> MESGIDLQGQFISALQSLGLSHDLAKLLWLPLPMLMMLIVATVGVLVAVWLERKISAAVQQRIGPEYIGPLGILAPLADGLKLIFKEDVLPANSDRWLFTLGPAVVVIPVFLSYIIVPFGQNLLISNLAMGVFLWIALSSIAPIGLLMAGYASNNKYSLLGGLRAAAQSISYEIPLALAVLAVAMMSNGLGTVEIVEQQSQYGILSWNVWRQPIGFLVFWIAALAECERLPFDLPEAEEELVAGYQTEYAGMKFALFYLGAYVNLVLSALLVSVLYFGGWSFPIPLETIANLLGVSETNPFLQIAFAVLGITMTLIKAYFFVFLAILLRWTVPRVRIDQLLDLGWKFLLPVGLVNLLLTAGLKLAFPVAFGG;> MDLVTLAGQLNAGTILPETILIVTLLVVLLADLIQGRQADRWTPYFAIVGLGGAIATMIPLWTQPATISFFGSFISDHLSLFFRGLIALSALGTILMSIRYVEQTGSSLGEFMTILLTATVGGMFIAGAQELVFIFVALETLSIASYLLTGYTKRDSRSNEAALKYLLIGAASSAIFLYGSSLLYGLSGGHTQLPAIAQALSSESLGLVVALVFVIAGISFKISAVPFHQWTPDVYEGAPTPVVAFLSVGSKAAGFALAIRFLTLAFPSVTDQWQLIFTVLAILSMILGNVVALAQTSMKRMLAYSSIGQAGFVMIGFVVGTEAGYASMLFYLLVYLFMNLGAFTCVILFSLRTGTDQISEYAGLYQKDPLLTLGLSLCLLSLGGIPPLAGFFGKIYLFWAGWQAGAYGLVLLGLLTSVISIYYYIRVVKMMVVKEPQEMSEAVRNYPEVSWSSFGLRPLQVGLVMTVIATSLAGILANPLFNLVNTAVWDVPQLANQPTVMEVAYQALSPAGKS;> MVAIPRLRDTATVFVLSGYEYFLGFLIICSLVPVLALAASALLRPKSGRMIRLTTYESGMEPIGGAWIQFNVRYYMFALVFVIFDVETVFLYPWAVAFHQLGLLAFIEALIFIAILVVALVYAWRKRALEWS;> MSTFPWLTTIILFPIVAALAIPFIPDPTGKGRPIRWYALAVGLIDFALIVYAFTNFYDLNTPGMQLWESYDWIPEIGLRWSVGADGLSMPLILLTGFITTLAILAAWPVTLKPRLFYFLMLAMYGGQIAVFAVQDMLVFFLAWELELIPVYLLLAIWGGHKRQYAATKFILYTAGSSLFILVAGLAMAFYGDTVSFDMQTLAAKDYALGFQLLVYAGFLVAYGVKLPIVPLHTWLPDAHGEATAPVHMLLAGILLKMGGYALIRMNVDMLPAAHAKFAPVLVILGVVNIIYAALTSYAQRNLKRKIAYSSISHIGFVLIGIASFTNLGMSGAVLQMVSHGLIGASLFFLVGATYDRTHTLILEEMGGVGQKMKKIFAMFTACSLASLALPGMSGFVAELMVFIGFATSDAYSLPFRVIVVFLAAVGVILTPIYLLSMLREIFYGPENKELVEHEALVDAEPREVFIIACLLVPIIGIGLYPKLLTQIYDATTGQVIARAREVLPTLAQQTEQPLGILPMVAPQLKANAQ;> MQLTYVLILAALLFCIGIYGLVTSRNAVRVLMSIELLLNAVNLNLIGFANYLDGQQIKGQVFAVFVITVAAAEAAVGLAIILAIYRNRDTVDMEKFNLLKW;> MEPLYQYAWLIPVLPLLGALIVGFGLIAFSETTSKLRRPSAIFIMALMAIAMGHSLTLFWSQVQGHLPYTQMIEWAAAGNLHIAMGYVIDPLAALMLVIVTTVAFLVMLYSDGYMAHDPGYVRFFAYLSLFGSSMLGLVVSPNLVQVYIFWELVGMCSYLLIGFWYDRKSAAEAAQKAFVTNRVGDFGLLLGMVGLFWATGTFDFAGMGDRLTELVNTGLLSPSLAAILAILVFLGPVAKSAQFPLHVWLPDAMEGPTPISALIHAATMVAAGVFLIARMFPVFEQLPQVMTTIAWTGAFTAFMGATIAITQNDIKKSLAYSTISQLGYMVMGMGVGAYSAGLFHLMTHAYFKAMLFLGSGSVIHSMEGVVGHNPDLAQDMRYMGGLRKYMPITGATFLVGCLAISGVPPFAGFWSKDEILGAVFHANPAMWLLTWLTAGLTAFYMFRMYFMTFEGKFRNVPPERQEHHDHHSHHAAVPHESPWTMTLPLVVLAIPSTLIGFVGTPFNNLFEVFIHAPGEEKVAEHAVDLTEFLILGGSSVGIGLMGITVAYLMYLKGTPSPQAIAKAIQPLYQFSLHKWYFDELYEAVFIKGCRRLARQVLEVDYNVVDGVVNLTGFVTMVTGEGLKYLQNGRAQFYALIVLLAVLGFVIFSVQT;> MDLATLTQTITFFALAAAVIIAALGVVLLDNVVYSAFLLGGVFLSIAGLYILMNADFVSAAQILIYVGAVNVLILFAIMLVNKRETYTPVPGRWLRQGGAAVVSLGVFALLTKMILQTPWQLSSVPPTPDSITTIGQHFFSDFLLPFELASVLLLMALIGAVVLARRELVLEPEPILGEEVVPPLELPERPREPVALSEK;> MPKIETRTEPMVINMGPHHPSMHGVLRLMVTLDGEDVIDCEPVIGYLHRGMEKIAENRTNIMFIPYVSRWDYAAGMFNEAVTVNAPEKLAGIPVPKRASYIRVIMLELNRIANHLLWLGPFLADVGAQTPFFYIFREREYIYDLFEAATGMRFINNNYFRIGGVAADLTYGWVTKCRDFCDYFLPKVDEYERLITNNPIFVRRLQGVGKISREEAINWGLSGPMLRASGVKWDLRKVDHYECYDDFDWDVPVATEGDCLARYIVRIQEMRESVKIIRQALDGLPGGPYENLEAKRMLEGAKSEWNGFDYQYIGKKLSPTFKIPKGEHYVRVESGKGELGIYLIGDDNVFPWRWKIRPPDFNNLQVLPQLLKGMKVADIVAILGSIDVIMGSVDR;> MKFLNQITNYAKEAVQSAKYIGQGLSVTFDHMRRRPITVQYPYEKLIPSERFRGRIHFEFDKCIACEVCVRVCPINLPVVDWVFNKELKKKELKHYSIDFGVCIFCANCVEYCPTNCLSVTEEYELATYDRHELNYDSVAMGRIPYKVTQDPMVTPIREFAYLPAGVMSGHDLPAGAQRAGERPEAIANTAKSSEN;> MSDTPEAPIVEAGPVGRLLQSQNLSVESLGRDASGVEMIKVDRDRLLAVCQTLYADGFNYLRCQAAYDSGPGQDLVSTYHLIKLSDNADRPPEVRIKVFVPRDDPRVPSVYWIWKTADWQERESYDMFGIVYEGHPNLKRILMPEDWVGWPLRKDYITPDFYELQEAY;> MTNTTSPAILNPIARPEVPQELAENIILTSLNDVYDWARLSSLWPLMYGTACCFIEFAAMIGSRFDFDRFGLVPRNSPRQADLIITSGTITMKMAPALVRLYEQMPSPKYVIAMGACTITGGMFSSDSYSAVRGVDKLIPVDVYLPGCPPRPEAIMDAIVKLRKKIANEHINERGNLAQTHRLFTAKHKMKPVPPILTGQYLNAPSRQAPPPALAAAMGIAVPALGEAVSETTSVAE;> MAVSTELLVLGVYGALAGLYLLVVPAIVYAYLNARWYVASSFERAFMYFLVTFFFPGLLLLAPFINFRPQPRSLNS;> MLLKSTTRHVHIYAGHVVDGEVHPDTETLTLNVDPDNELEWNEAALAKVEAKFRELVANAAGEDLTEYNLRRIGSDLEHFIRSLLMQGEIGYNLNSRVRNYSLGIPRVNHS;> MGLLAGYQFVKDLESAGALALFVPPEGGFEGRYQRRLRSKGYTTLPMSAPGLGDLAAYLTQEHGIRPAHTGKEDIRVYFQPPLVTYHLENLPPNAKGLVLWLIDGKRLSKQEFAYLAQLTQTLPKFKVVVEVGGDRVVRWEPLADWVAAA;> MAIKKGDLVKVVAEKLANSLEALASDHRYPPYLFEGRGEVVDIRGDYAQIKFPVPTPTVWLRLDQLEVAQ;> MDAVISVKPILLAMTPVFILLCLFFGTRNGFYDTDQYHGNGSAH;> MATDFNRGIMKFDGADSPAMIAISAVLILGFIAALIWWALHTAYA;> MIRPIADTYPLLPLSKAQMGQRQEIINSHKRLWDKTMATDLIMTILPGMTVKVTNPNDTYYQFQGIVQRITDGKVAVLFEGGNWDKLVTFQASELEPVVVTPKEKAKAKK

In both cyanobacteria and plants, a type-I NAD(P)H dehydrogenase-like (NDH-1) complex is crucial for CEF and respiration. The NDH-1 complexes belong to the NAD(P)H:Quinone oxidoreductase family that includes the complex I (NADH dehydrogenase) of the respiratory chain in bacteria and mitochondria. The electron delivered from Fd is eventually transferred to PQ which is bound within the NDH complex. To further advance our understanding of NDH functionality, we solved two single particle cryo-electron microscopy (cryo-EM) structures of NDH-1L from T. elongatus BP-1.

We first solved the structure of NDH-1L complex purified from T. elongatus BP-1 at an overall resolution of 3 Å. Interestingly, we found that the NDH-1L complex binds a PQ molecule at a pocket above the membrane plane. We assume that this is an endogenous PQ molecule, which was trapped in the cyanobacterial NDH-1L complex during purification, as was earlier reported for Escherichia coli complex I40. Thus, we named this structure as NDH-PQ. Similar to the two previously reported cyanobacterial NDH-1L structures, our NDH-PQ structure also contains 18 subunits, without any signs of association with NdhV. In addition, we found that the NdhS subunit in the NDH-PQ structure exhibits weak cryo-EM density, suggesting that NdhS is also loosely associated. In the NDH-PQ structure, we modeled a PQ molecule in a pocket (PQ chamber) at the interface of the membrane and hydrophilic arms. The smaller PQ chamber is caused by the different conformation adopted by the β1-2 loop of NdhH, which intrudes into the PQ chamber, and the side chain of M22 blocks the path between PQ and the N2 cluster. Indeed, the H23-D124 hydrogen bond is preserved in our NDH-PQ structure; however, the PQ molecule is more distantly located from the N2 cluster, without direct linking with NdhH-Y72 and NdhH-H23, implying that our structure represents a state of NDH/complex I that is not fully active. The occluded feature of the PQ chamber, together with the long distance between PQ and the N2 cluster, implies that our structure represents an idle state of the NDH complex, as was previously suggested for the Yl complex I39.> APEDPSDLLQHVKFQSSNFENILTWDSGPEGTPDTVYSIEYKTYGERDWVAKKGCQRITRKSCDLTVETGDLQELYYARVTAVSAGGRSATKMTDRFSSLQHTTLKPPDVTCISKVRSIQMIVHPTPTPIRAGDGHRLTLEDIFHDLFYHLELQVNRTYQMHLGGKQREYEFFGLTPDTEFLGTI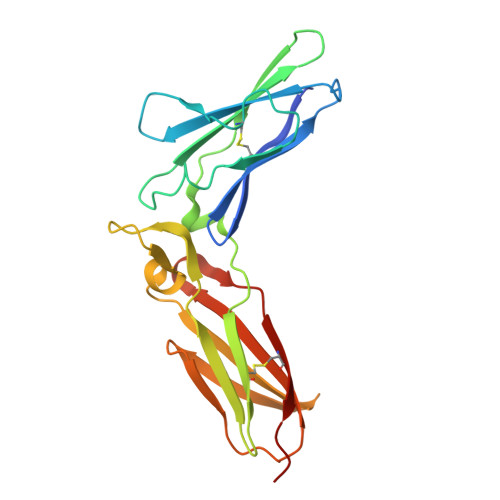MICVPTWAKESAPYMCRVKTLPDRT The 8.8a-oleandolide epoxygenase OleP, from Streptomyces antibioticus, is the P450 involved in the polyketide biosynthesis of the antibiotic oleandomycin. It introduces an epoxide function to the C8-C8a of the macrolactone ring of two structurally different intermediates, namely the aglycone 8.8a-oleandolide (DEO) and the C3-mono-glycosylated L-olivosyl-8.8a-deoxyoleandolide (L-O-DEO). Substrate binding to the cytochrome P450 OleP is coupled to a large open-to-closed transition that remodels the active site, minimizing its exposure to the external solvent. When the aglycone substrate binds, a small empty cavity is formed between the I and G helices, the BC loop, and the substrate itself, where solvent molecules accumulate mediating substrate-enzyme interactions.

As predicted, the substitution of G92 with a tryptophan and S240 with a tyrosine resulted in filling the solvent cavity, which is occupied by the bulky aromatic sidechains. This reduces to some extent the volume of the active site in both mutants, which is ~606.7 Å3 in the wild type and ~582.5 and ~566.8 Å3 in G92W and S240Y, respectively. In G92W and S240Y mutants, the bulkier and more hydrophobic groups are located in the cavity, causing, respectively, the partial and the total displacement of the solvent molecules and resulting in the formation of direct interactions between the enzyme and the substrate. Within the solvent cavity, the aromatic side chain of S240Y and G92W form additional direct and directional contacts with the substrate and with other residues within the distal pocket, inducing the partial or the total removal of solvent molecules from that region. The insertion of a tryptophan in position 92 and of a tyrosine in position 240 also generate additional contacts within the protein structure, involving residues located in the active site of the enzyme. The superposition of the modeled open structure onto the crystallographic closed complex suggests that the presence of a tyrosine at position 240 would jeopardize the enzyme closure since its repositioning could lead to a collision with the BC loop at residues 91–93. Indeed, while the effect of the ionic strength on the spin state equilibrium of the wild type and E89Y is comparable, showing the total low-to-high spin shift at I = 2.5–3 M, in G92W and S240Y mutants the shift is not complete even at the highest ionic strength conditions tested (I = 3.5 M). Therefore, at physiological ionic strength conditions, substrate binding to G92W and S240Y mutants cannot trigger the structural transition that induces the displacement of the water molecule from the sixth coordination position of the iron and the spin-state shift, not even on a partial population of the enzyme, as it occurs in the case of wild type and E89Y variants. On the other hand, in crystals obtained at higher ionic strength (I ~4.4 M), we observed only closed monomers of the complex for all mutants.

>[6x]AATHTGPTPADAVPAYPFSLPHALDLDPHYAELRRDEPVSRVRLPYGEGTAWLVTRMSDARIVLGDSRFSTAAATDPATPRMFPTPPEPDGVLAQDPPDHTRLRRLVGKAFTARRVEEMRPRVRSLVDSLLDDMVAHGSPADLVEFLAVPFPVAVICELLGVPLEDRDLFRTFSDAMLSSTRLTAAEIQRVQQDFMVYMDGLVAQRRDAPTEDLLGALALATDNDDHLTKGEIVNMGVYLLIAGHETSVNQITNLVHLLLTERKRYESLVADPALVPAAVEEMLRYTPLVSAGSFVRVATEDVELSTVTVRAGEPCVVHFASANRDEEVFDHADELDFHRERNPHIAFGHGAHHCIGAQLGRLELQEALSALVRRFPTLDLAEPVAGLKWKQGMLIRGLERQIVSW> MGSDKIHHHHHHMTKQSKTQIRICFVGDSFVNGTGDPECLGWTGRVCVNANKKGYDVTYYNLGIRRDTSSDIAKRWLQEVSLRLHKEYNSLVVFSFGLNDTTLENGKPRVSIAETIKNTREILTQAKKLYPVLMISPAPYIEQQDPGRRRRTIDLSQQLALVCQDLDVPYLDVFPLLEKPS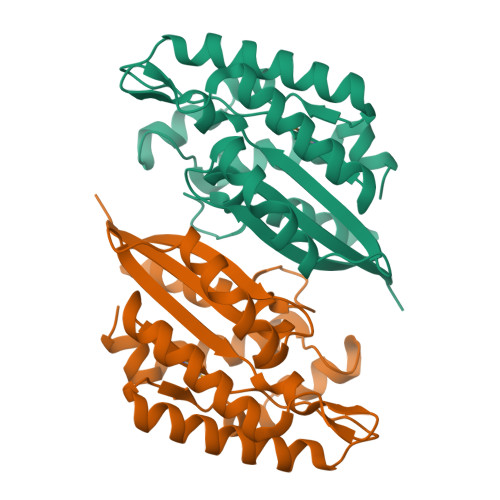VWLHEAKANDGVHPQAGGYTEFARIVENWDAWLNWFR> DPISNAIENAVSTLADTTISRVTAANTAASSHSLGTGRVPALQAAETGASSNASDENLIETRCVMNRNGVNEASVEHFYSRAGLVGVVEVKDSGTSQDGYTVWPIDVMGFVQQRRKLELSTYMRFDAEFTFVSNLNDSTTPGMLLQYMYVPPGAPKPDGRKSYQWQTATNPSIFAKLSDPPPQVSVPFMSPASAYQWFYDGYPTFGEHKQATNLQYGQCPNNMMGHFAIRTVSESTTGKNVHVRVYMRIKHVRAWVPRPFRSQAYMVKNYPTYSQTISNTAADRASITTTDYEGGVPANPQRTF;> SPSVEACGYSDRVAQLTVGNSTITTQEAANIVLSYGEWPGYCPSTDATAVDKPTRPDVSVNRFYTLSTKSWKTESTGWYWKFPDVLNDTGVFGQNAQFHYLYRSGFCMHVQCNASKFHQGALLVVVIPEFVVAASSPATKPNGQGLYPDFAHTNPGKEGQVFRDPYVLDAGIPLSQALVFPHQWINLRTNNCATIIMPYVNALPFDSALNHSNFGLAVIPISPLKYCNGATTEVPITLTIAPLNSEFSGLRQAIKQ;> GLPTELKPGTNQFLTTDDGTSPPILPGFEPTPLIHIPGEFTSLLDLCRIETILEVNNTTGTTGVNRLLIPVRAQNNVDQLCASFQVDPGRNGPWQSTMVGQICRYYTQWSGSLKVTFMFTGSFMATGKMLIAYTPPGSAQPTTREAAMLGTHIVWDFGLQSSVTLVIPWISNTHFRAVKTGGVYDYYATGIVTIWYQTNFVVPPDTPSEANIIALGAAQENFTLKLCKDTDEIRQTAEYQN;> GAQVSAQKSGTHETGNIATEGSTINFTNINYYKDSYAASASRQDFTQDPTKFTSPVLDAIKEAAAPLQ

Coxsackievirus A6 (CV-A6) has recently overtaken enterovirus A71 and CV-A16 as the primary causative agent of hand, foot, and mouth disease worldwide. To initiate infection, enterovirus particles progress through a set of distinct functional intermediates: the infectious native virion expands into a destabilised altered or A-particle, in which the internal capsid protein VP4 has been displaced. The genome is released through a capsid opening, leaving the empty capsid as the non-infectious end product. The major capsid proteins VP1, VP2, and VP3 are arranged with pseudo-T = 3 icosahedral symmetry with VP1 subunits forming pentamers around the fivefold axes and VP2 and VP3 forming heterohexamers around the threefold symmetry axes of the capsid.

We show that the CV-A6 virion has features characteristic of virions of other enteroviruses, including a compact capsid, VP4 attached to the inner capsid surface, and fatty acid-like molecules occupying the hydrophobic pockets in VP1 subunits. The structure of the CV-A6 virion was determined to a resolution of 2.68 Å, whereas those of the altered and empty particles reached resolutions of 2.50 and 2.82 Å, respectively. Unlike the altered and empty particles, the CV-A6 virion does not contain openings located on the twofold symmetry axes of its capsid. The maximum radius of the CV-A6 virion is 161 Å. The cryo-EM reconstruction enabled the building of residues 9 to 300 of 304 of VP1, 7 to 256 of 256 of VP2, the complete structure of 241 residues of VP3, and residues 15 to 69 of 69 of VP4. The pocket of CV-A6 contains an elongated density (pocket factor), which we modelled as C-18 stearic acid in accordance with the length of the electron density in the locally sharpened and masked map. The cryo-EM density of the stearic acid in CV-A6 is discontinuous in the sharpened map, whereas it is well-defined and continuous in the locally sharpened map but has lower density values than the surrounding protein structure, indicating possible flexibility of the pocket factor, variability in the type of the molecule, or lower than 100% occupancy. The cryo-EM map of the CV-A6 virion contains an elongated continuous density positioned parallel to the N-terminal segment of VP4. We speculate that this density corresponds to myristate attached to an N-terminal glycine of VP4. The side chain of Trp38 of VP2 interacts at a distance of 4.6 Å with a density disc that is connected to the elongated curved putative RNA density positioned next to a twofold axis.>[2x]GSGGIEGRHMVELLKLVRSSGCAAKVGPGDLQEILKGFNIYTDESTLVSIGDDAGVYEHNGIIWVYTVDIITPVVNDPYLWGAISTANALSDVYAMGGIPVNALAISCFNNCELDIEIFREVIRGALDKLREAKTVLLGGHTIDDKEPKFGLSVAGICPEGKYITQSGAQVGQLLILTKPIGTGILIKGLKEGILKEEDINEAIENMLA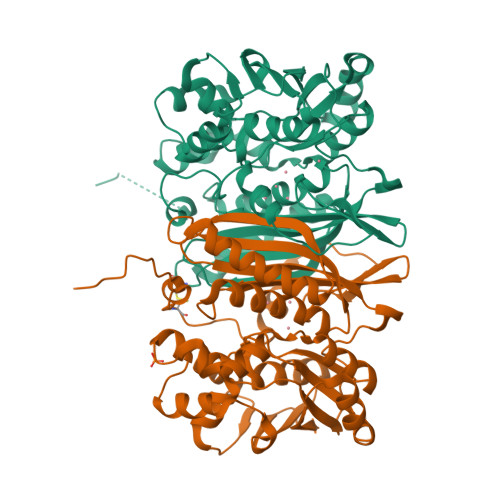LNDKARNLMLSLDATACTDVTGFGLLGHAWNICKNSNIGARIFFEKVPYYQLSENLVKKKIYPKGAIENLNFVKNYLKSNLDNWKLILLSDPVTSGGLLFTINKEKLEKIDETAKELEVNYWIIGETIAENVLEVL> MVKYEDKICLYNAKGELVEENVPLEAISPLYNPTIQKLVKDIKRTVAVNLAGIENALKTGAVGGKACVIPGRTLDLPIVENAETIMEYVDKLLRISPDDDTSVKLINDGKQMAVQLPSKRLEVAAEYSISMLNTAMALKEAIIKTFDVDMFDAPMVHAAILGRYPQVPDYMGANIASL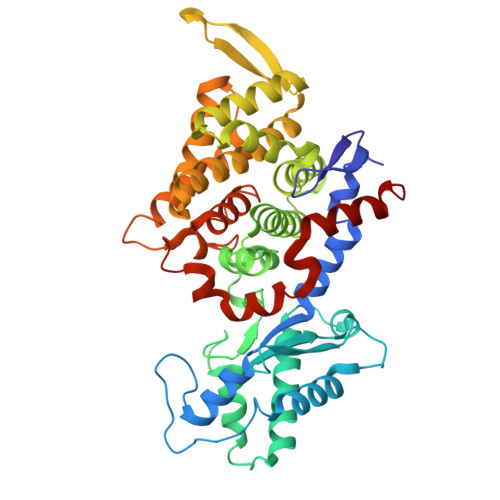LGAPTNLEGLGYALRNIMVNHYVATTKKNIMNAVAFASIMEQTAMFEMGDAIGSFERLHLLGLAYQGLNADNLVIDLVKANGKNGTVGTVVASIVERALEDGVITEDKKMPSGFVLYKPVDVAKWNAYAAAGLVAAVIVNCGAARAAQNVASTILYYNDIIEYETGLPGVDFGRAEGTAVGFSFFSHSIYGGGGPGIFNGNHIVTRHSKGFAIPPVCAAMCVDAGTQMFSPEKTSALVGAVFSAIDEFREPLKYVIDGALAVKDKI> SSQIRQNYSTDVEAAVNSLVNLYLQASYTYLSL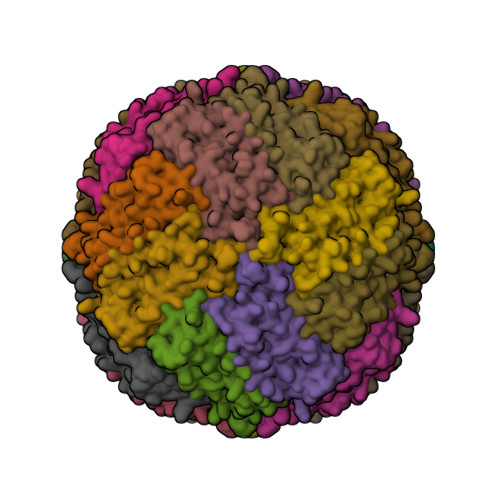GFYFDRDDVALEGVSHFFRELAEEKREGYERLLKMQNQRGGRALFQDIKKPAEDEWGKTPDAMKAAMALEKKLNQALLDLHALGSARTDPHLCDFLETHFLDEEVKLIKKMGDHLTNLHRLGGPEAGLGEYLFERLTLKH>MVPGACPLILRLSPTLHSADLIRDIDAMRWFLFEDTGVPLPEVNIEVLPEPTEKLTVLLYQEPVFSLSIPAQADYLLIGADASVVGDSQTLPNGMGQICWLTKDMAHKAQGFGLDVFAGSQRISALLKCVLLRHMGEFIGVQETRYLMNAMEKNYSELVKELQRQLPINKIAETLQRLVSERVSIRDLRLIFGTLIDWAPREKDVLMLTEYVRIALRRHILRRLNPEGKPLPILRIGEGIENLVRESIRQTAMGTYTALSSRHKTQILQLIEQALKQSAKLFIVTSVDTRRFLRKITEATLFDVPILSWQELGEESLIQVVESIDLSEEELADNEE[18x]

The inner membrane export gate protein, SctV (InvA in SPI-1 and SsaV in SPI-2), is the largest component of the injectisome and is essential for assembly and function of T3SS. SctV comprises a highly conserved N-terminal transmembrane (TM) domain and a less conserved C-terminal cytoplasmic domain (SctVC), which are connected via a ∼20–40 amino acid linker, SctVL, in most bacteria using the T3SS. It has been reported that SctV is one of the “engines” of T3SS; the TM domain forms a putative proton channel, and SctVC forms a nonameric ring connecting to SctN (ATPase) through SctO (the stalk protein) to function as the F0F1-ATPase, coupling energy from ATP hydrolysis and the proton-motive force to secrete unfolded bacterial effectors into the eukaryotic host. Consistent with other reported SctVC structures, the SsaVC monomer also has a four-subdomain (SD) structure and further assembles to a nonameric ring aligned to SD3, which is the most conserved region of SsaVC.

Unlike InvAC, SsaVC could maintain a very stable high oligomeric state even in the high salt concentration analyzed by the size exclusion chromatography (SEC) and dynamic light scattering (DLS). Through a cryo-EM single particle analysis approach, we reconstructed and classified two conformations of SsaVC: one 3.55 Å cryo-EM structure with double stacked nonameric rings with D9 symmetry, and the other 3.64 Å cryo-EM structure with a single nonameric ring with C9 symmetry, the particle number of which are approximately comparable. The double-layer ring conformation of SsaVC is considered to be an artifact, consistent with a previous study. Notably, most of the C9 single-layer ring of the SsaVC particles were calculated from top views, and most of the D9 double-layer ring of SsaVC particles came from side views. We speculate that this is because the top-view protein particles are more vulnerable to air–water interface damage than the side-view particles.> QGRKIFKVFNQDFIVDERYTVTKELGQGAYGIVCAAVNNQTSEGVAIKKVTNVFSKKILAKRALREIKLLQHFRGHRNITCLYDMDIPRPDNFNETYLYEELMECDLAAIIRSGQPLTDAHFQSFIYQILCGLKYIHSANVLHRDLKPGNLLVNADCELKICDFGLARGFSVDPEENAGYMTEYVATRWYRAPEIMLSFQSYTKAIDVWSVGCILAELLGGRPFFKGRDYVDQLNQILHILGTPNEETLSRIGSPRAQEYVRNLPFMAKKPFPTLFPNANPDALDLLDRMLAFDPSSRISVEQALEHPYLHIWHDASDEPDCPTTFNFDFEVVEDVGEMRKMILDEVYRFRQLVRTAPGAGGHGAPHAPQVPIPAGAGQGQWKAEDPRPQEYVGQMNDLEAELAGGLD

Fungal proteins that function during the infection process might be potential candidates, and Mps1 (M. oryzae mitogen-activated protein kinase 1) is such a protein that plays a critical role in appressorium penetration of the plant cell wall. Mps1 plays a role in appressorium penetration and invasive hyphal growth periods but does not influence the formation of appressoria. As a typical kinase, the overall structure of Mps1 can be divided into two domains, a smaller N-terminal lobe (N-lobe, residues Q5 to E104) and a larger C-terminal lobe (C-lobe, residues C109 to D412), with a hinge region (residues E105 to E108) connecting them. The deep cleft between the N-lobe and the C-lobe serves as the catalytic pocket for binding the cosubstrate ATP and substrates.

Cocrystallization of A378-0 with Mps1 revealed that A378-0 binds to the catalytic pocket of Mps1, while the three ring-type substructures of A378-0 constitute a triangle that squeezes into the pocket. The structure was determined at a 2.15-Å resolution. Structural superimposition with apo-Mps1 shows a root mean square deviation (RMSD) of 0.311 Å, indicating that only subtle conformational changes occurred in the newly determined structure. A378-0 exhibits a compact conformation for squeezing into the pocket: the indole ring is oriented perpendicular to the central 1,6-naphthyridine ring, the benzene ring tilts about 45° from the 1,6-naphthyridine ring, and thus, the planes of the three rings approximate an equilateral right triangle. There are seven intermolecular hydrogen bonds between A378-0 and Mps1. Residues G30 and Q31 belong to the glycine-rich loop (G-loop) between strands β1 and β2 of Mps1, and the formation of the two hydrogen bonds results in an extension of the β1-strand compared with apo-Mps1. Second, one nitrogen atom of the 1,6-naphthyridine ring interacts with the main-chain oxygen of residue M107 of the hinge region of Mps1, which leads to a conformational change of the hinge and the emergence of the β6-strand compared with apo-Mps1. Third, amide group I of A378-0 uses its oxygen atom to interact with the side chain nitrogen of residue K52 of the β3-strand of Mps1, while amide group II of A378-0 uses its nitrogen atom to interact with the side chain oxygen of residue D167 of the DFG motif of Mps1, rendering stabilization of residue D167 to point inward, i.e., Mps1 in the “DFG-aspartate-in” state (the side chain of the aspartate of the DFG motif points to the cleft). Finally, the last two hydrogen bonds occur between the nitrogen atom of the indole ring of A378-0 and the two oxygen atoms of the side chain carboxyl group of residue E70 of Mps1, which stabilizes the αC-helix in the “αC-helix-in” conformation (the side chain of the glutamate of the αC-helix points to the cleft). Besides hydrogen bonds, hydrophobic interactions also function in stabilizing A378-0 in the cleft between the N- and C-lobes of Mps1.In the Fo sector, eight to 15 copies of subunit c are assembled into a closed ring, which rotates around its axis as ions permeate across the enzyme. The c-ring harbors a series of identical ion-binding sites, typically one per c-subunit, which selectively recognize the coupling ion. We describe the structure of a novel type of Na+-binding site in the c-ring of the F1Fo-ATP synthase from F. nucleatum and demonstrate that this enzyme is physiologically coupled to the SMF. The c-ring features two glutamate residues in each of its 11 ion-binding sites, instead of a single carboxylate side-chain as is typical.

Crystals of the c11 ring were first grown at pH 5.3 and one of the crystals yielded a complete 2.2 Å dataset. In this crystal, one asymmetric unit contains two complete c-rings. The c-ring was crystallized in the presence of near-physiological concentrations of Na+ (100 mM). To confirm the location of the Na+-binding sites, we calculated an omit electron-density map. This map reveals 11 binding sites, each located at one of the interfaces between c-subunits. The most notable difference is the presence of a second glutamate side-chain, Glu32, in addition to the conserved Glu on the C-terminal helix (Glu65). Both side-chains contribute to Na+ coordination, via one oxygen atom of each carboxyl group. The other two oxygen atoms are at hydrogen-bonding distance of ∼2.7 Å from each other. This arrangement suggests that a proton is bound to the site in addition to Na+, consistent with the free-energy calculations described above. In addition to Glu32 and Glu65, Ser66:Oγ and Val63:O from the adjacent c-subunit also contribute to Na+ coordination. Ser66:Oγ and Tyr70:OH also interact with Glu65, as hydrogen-bond donors, stabilizing the so-called ion-locked conformation of the site.

>[22x]MDLLTAKTIVLGCSAVGAGLAMIAGLGPGIGEGYAAGKAVESVARQPEARGSIISTMILGQAVAESTGIYSLVIALILLYANPFLSKLG5-(4-fluorophenyl)-2,3-dihydroxy-N-[3-(pyrrolo[3,2-c]pyridin-1-ylmethoxy)propyl]benzamide 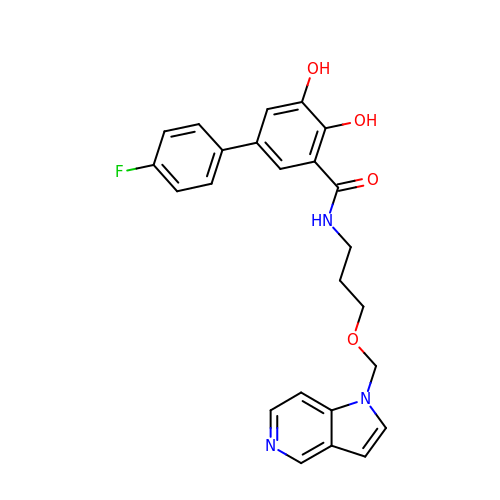| C24 H22 F N3 O4 | RWYTVUVWQHASIX-UHFFFAOYSA-N> GPLHMGSSEESQAFQRQLTALIGYDVTDVSNVHDDELEFTRR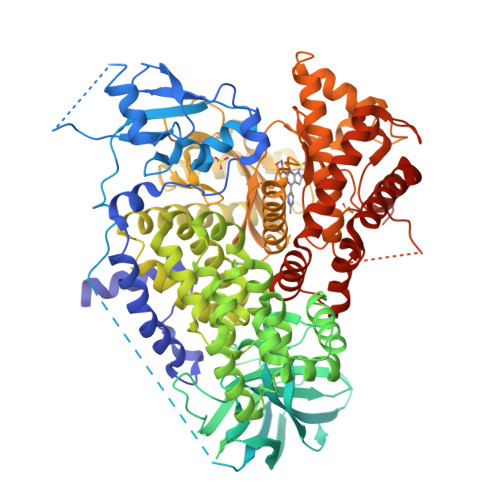GLVTPRMAEVASRDPKLYAMHPWVTSKPLPEYLWKKIANNCIFIVIHRSTTSQTIKVSPDDTPGAILQSFFTKMAKKKSLMDIPESQSEQDFVLRVCGRDEYLVGETPIKNFQWVRHCLKNGEEIHVVLDTPPDPALDEVRKEEWPLVDDCTGVTGYHEQLTIHGKDHESVFTVSLWDCDRKFRVKIRGIDIPVLPRNTDLTVFVEANIQHGQQVLCQRRTSPKPFTEEVLWNVWLEFSIKIKDLPKGALLNLQIYCGKAPALSSKASAESPSSESKGKVQLLYYVNLLLIDHRFLLRRGEYVLHMWQISGKGEDQGSFNADKLTSATNPDKENSMSISILLDNYCHPIALPKHQPTPDPEGDRVRAEMPNQLRKQLEAIIATDPLNPLTAEDKELLWHFRYESLKHPKAYPKLFSSVKWGQQEIVAKTYQLLARREVWDQSALDVGLTMQLLDCNFSDENVRAIAVQKLESLEDDDVLHYLLQLVQAVKFEPYHDSALARFLLKRGLRNKRIGHFLFWFLRSEIAQSRHYQQRFAVILEAYLRGCGTAMLHDFTQQVQVIEMLQKVTLDIKSLSAEKYDVSSQVISQLKQKLENLQNSQLPESFRVPYDPGLKAGALAIEKCKVMASKKKPLWLEFKCADPTALSNETIGIIFKHGDDLRQDMLILQILRIMESIWETESLDLCLLPYGCISTGDKIGMIEIVKDATTIAKIQQSTVGNTGAFKDEVLNHWLKEKSPTEEKFQAAVERFVYSCAGYCVATFVLGIGDRHNDNIMITETGNLFHIDFGHILGNYKSFLGINKERVPFVLTPDFLFVMGTSGKKTSPHFQKFQDICVKAYLALRHHTNLLIILFSMMLMTGMPQLTSKEDIEYIRDALTVGKNEEDAKKYFLDQIEVCRDKGWTVQFNWFLHLVLGIKQGEKHSA>MPMTDLPSAVTNERTEQTNTTNEQQESKGFDYLIVGAGFAGSVLAERLASSGQRVLIVDRRPHIGGNAYDCYDDAGVLIHPYGPHIFHTNSKDVFEYLSRFTEWRPYQHRVLASVDGQLLPIPINLDTVNRLYGLNLTSFQVEEFFASVAEKVEQVRTSEDVVVSKVGRDLYNKFFRGYTRKQWGLDPSELDASVTARVPTRTNRDNRYFADTYQAMPLHGYTRMFQNMLSSPNIKVMLNTDYREIADFIPFQHMIYTGPVDAFFDFCYGKLPYRSLEFRHETHDTEQLLPTGTVNYPNDYAYTRVSEFKHITGQRHHQTSVVYEYPRAEGD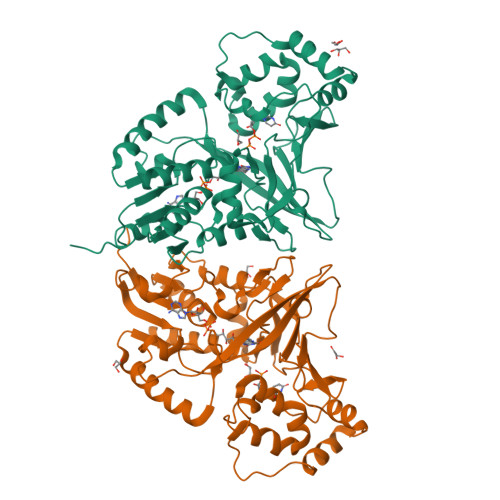PYYPVPRPENAELYKKYEALADAAQDVTFVGRLATYRYYNMDQVVAQALATFRRLQGQPEQGNAE[10x]>[6x]MKIYRPLWEDGAFLMPQQFQQQAAWDVHLADSVARMGLAHPWGVVAAEFDDSLLPLSRLNATRLIVRFPDGTLIDTERADNLPPVCDLSTVSDRSLVDIVLALPLLNANGGNLDNGSESERPRRWKSERVNVQELAGHEQSEVAVLRHNLTLRMAHQENAAWLTCPVTRLVRDAQGQWCRDPRFIPPLLTLSASPSLMTELAELLHHLQARRQRLMSMRRENNARLADFAVADVSLFWLLNALNSAEPVLKELLDMPYRHPELLYRELARLAGSLLTFSLEHNVDAVPAYHHETPENVFPPLLSLLNRLLEASLPSHHHHHH;> MGFPASEIKDAVIPEESHLPPIVHVTFMGLYGVTSPLPAHYISDIAQQREGHEAAADFLDIFSHRLITQYYRIWRKYSYPATFEAGGQDKTSQYLLGLARLGIPGCAQNIATPVSRFLALLPLMLLPGRTAEGLTSLVTLLAPGTQARVWHHDRRRIPLKTPLTMRVHHPVSLKSRPVMGDHATDVNGQVLLQLSTQTGSEVQGWLPGGHLYSDLLALLHVYLGSRLDVRLQLCVERSLLPDARLSCRPAAGSPQLGRTAVMRTQAKIATSAARVMTISLGRYQRVQEHYQRKETQENGDYRW;>[2x]MDDLTLRYFDAEMRYLREAGKAFAQAHPDRAAMLDLDKAGTPDPCVERLFEGFAFSMGRLRQKIDDDLPELTESLVSMLWPHYLRTIPSLSVVALTPRLSVMKMAETVPAGLEVTSRPVGPGNTVCRYRTTRAIPLNPLAVEKVVMTTEPDGRSVLKIGFACSELADWSQVDLHRLSLYLAAEAPVSSTLHLMMTKRLAALYLRLPGNDERIRIDGWFSPGGFAEEDRLWPKGDSAFSGYQLLLEYFTFREKFMFVHLNGLENVSLPAGISGFDLEVVLSQPWPADLPVTDDALCLHCVPVINLFTLEADPLIINGLESEYLLRPKRLQDGYTEIYSVDAVTGSGRTGSAEYVPFTSFRHRGGMLRHDAPERYYHTRVKRGVTGMYDTWLILGGQRWEADRMPERETLSLRITGTNGQLPRRALQSTLLDRCEQVLQAPVSVRNLCKPTLPVYPPTEDRFHWRVMSHLGTGFLNMLSSAEVLRGTLALYNWRDDELNHRRLDAILAVQHHRIQRFEKGFLLRGLDVEVTLDGNGFAGEGDIHLFGEMLNRFLALYADMNQFNQLTLIVQPEGKCIRWKENHNPRLPG

Type VI secretion systems (T6SSs) are found in a broad range of Gram-negative bacteria and transport proteins directly into recipient cells. The T6SS needle oligomerizes in the bacterial cytoplasm and comprises an inner tube, made of Hcp hexameric rings arranged with helical symmetry, surrounded by TssB–TssC rings forming the sheath. Localization of the needle within a donor cell is mediated by a pre-assembled cytoplasmic baseplate comprising TssK, TssF, TssG, TssE, VgrG, and a PAAR-repeat protein. To address this knowledge gap, we report here the 3.7 Å resolution cryoEM structure of the EAEC TssK–TssF–TssG complex.

To understand the architecture of the T6SS baseplate, we overexpressed and purified an EAEC complex comprising full-lengh TssF and TssG (residues 64–366) as well as the shoulder and neck domains of TssK (TssKSN, residues 1–315). The final cryoEM map has an overall resolution of 3.7 Å (3.9 Å for the TssF–TssG focused map) and is best resolved for the region corresponding to TssK, TssG, and the C-terminal domains of TssF. The final model comprises TssK residues 1–315 (with a chain break between residues 220–230), TssF residues 45–587 (with a chain break between residues 393–404), as well as TssG residues 122–365 (with a chain break between residues 330–336,). The cryoEM map also contains a few unassigned densities that were modeled as polyalanine chains and which likely account for the N-terminal regions of TssF and TssG. Our results show TssG acts as an adaptor interacting with two TssK trimers and two TssF protomers to form part of a baseplate wedge (which also comprises TssE). The (TssF)2–(TssG)1 complex assembles as a locally pseudo-symmetrical heterotrimer with a 2:1 stoichiometry. The N-termini of the three modeled chains form a three-helix bundle interacting with a triangular core, which is formed upon trimerization of the C-terminal domains of TssF and TssG. Each TssKSN trimer attaches to one of the two extended loops protruding from the TssG C-terminal domain. Loop 1 anchors a TssK trimer near the apex of the pseudo-threefold symmetrical (TssF)2–(TssG)1 C-terminal triangle, whereas loop 2 binds another TssKSN trimer at the periphery of the triangle. The two TssK trimers are tilted ~ 60° relative to each other and interact together, burying an average surface area of 1000 Å2 at their interface.>GSQRVLVEPDAGAGVAVMKFKNPPVNSLSLEFLTE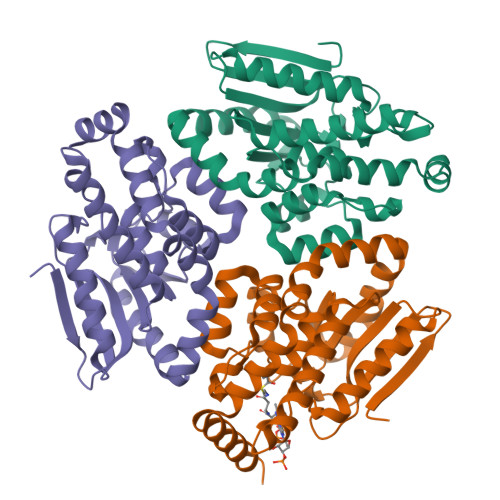LVISLEKLENDKSFRGVILTSDRPGVFSAGLDLTEMCGRSPAHYAGYWKAVQELWLRLYQSNLVLVSAINGACPAGGCLVALTCDYRILADNPRYCIGLNETQLGIIAPFWLKDTLENTIGHRAAERALQLGLLFPPAEALQVGIVDQVVPEEQVQSTALSAIAQWMAIPDHARQLTKAMMRKATASRLVTQRDADVQNFVSFISKDSIQKSLQMYLERLKEEKG[3x]>PHLRNRPGKGHNYIDGMTQEDATCKPVTYAGACSSFDVLLEKGKFPLFQSYAHHRTLLEAVHDTIIAKADPPSCDLQSAHGNPCMKEKLVMKTHCPNDYQSAHYLNNDGKMASVKCPPKYELTEDCNFCRQMTGASLKKGSYPLQDLFCQSSEDDGSKLKTKMKGVCEVGVQALKKCDGQLSTAHEVVPFAVFKNSKKVYLDKLDLKTEENLLPDSFVCFEHKGQYKGTMDSGQTKRELKSFDISQCPKIG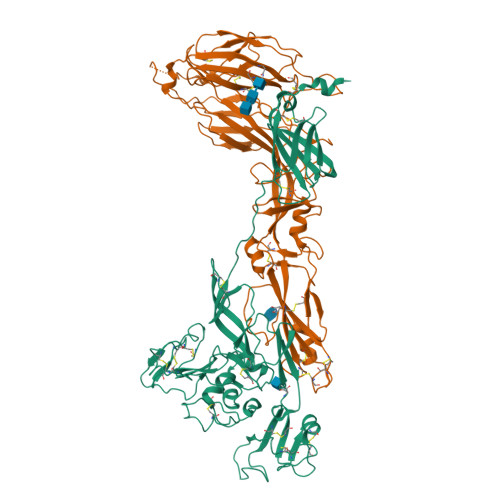GHGSKKCTGDAAFCSAYECTAQYANAYCSHANGSGIVQIQVSGVWKKPLCVGYERVVVKRELSAKPIQRVEPCTTCITKCEPHGLVVRSTGFKISSAVACASGVCVTGSQSPSTEITLKYPGISQSSGGDIGVHMAHDDQSVSSKIVAHCPPQDPCLVHGCIVCAHGLINYQCHTALSAFVVVFVFSSIAIICLAVLYRVLKCLKIAPRKVLNPLMWITAFIRWIYKKMVARVADNINQVNREIGWMEGGQLVLGNPAPIPRHAPIPRYSTYLMLLLIVSYASACSELIQASSRITTCSTEGVNTKCRLSGTALIRAGSVGAEACLMLKGVKEDQTKFLKIKTVSSELSCREGQSYWTGSFSPKCLSSRRCHLVGECHVNRCLSWRDNETSAEFSFVGESTTMRENKCFEQCGGWGCGCFNVNPSCLFVHTYLQSVRKEALRVFNCIDWVHKLTLEITDFDGSVSTIDLGASSSRFTNWGSVSLSLDAEGISGSNSFSFIESPGKGYAIVDEPFSEIPRQGFLGEIRCNSESSVLSAHESCLRAPNLISYKPMIDQLECTTNLIDPFVVFERGSLPQTRNDKTFAASKGNRGVQAFSKGSVQADLTLMFDNFEVDFVGAAVSCDAAFLNLTGCYSCNAGARVCLSITSTGTGSLSAHNKDGSLHIVLPSENGTKDQCQILHFTVPEVEEEFMYSCDGDERPLLVKGTLIAIDPFDDRREAGGESTVVNPKSGSWNFFDWFSGLMSWFGGPLKTILLICLYVALSIGLFFLLIYLGRTGLSKMWLAATKKASDYKDHDGDYKDHDIDYKDDDDK[2x]> MAAIQGIEGVISQLQATAMAARGQDTHSQSTVSFAGQLHAALDRISDRQAAARVQAEKFTLG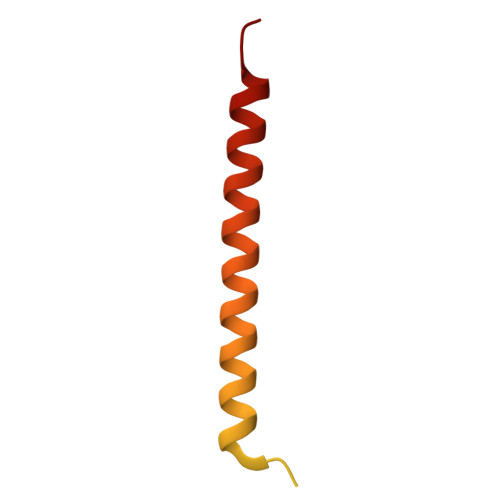EPGIALNDVMADMQKASVSMQMGIQVRNKLVAAYQEVMSMQV> MHHH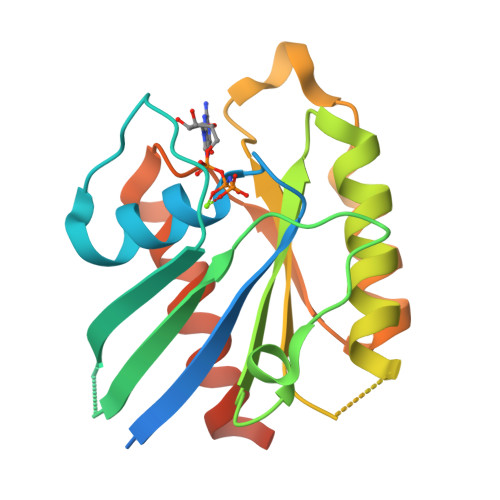HHHSSGRENLYFQGMPLVRYRKVVILGYRCVGKTSLAHQFVEGEFSEGYDPTVENTYSKIVTLGKDEFHLHLVDTAGQDEYSILPYSFIIGVHGYVLVYSVTSLHSFQVIESLYQKLHEGHGKTRVPVVLVGNKADLSPEREVQAVEGKKLAESWGATFMESSARENQLTQGIFTKVIQEIARVENSYGQERRCHLM Here we present rotamer inverted fragment finder–diffusion (Riff-Diff), a hybrid machine learning and atomistic modelling strategy for scaffolding catalytic arrays in de novo proteins. We highlight the general applicability of Riff-Diff by designing enzymes for two mechanistically distinct chemical transformations, the retro-aldol reaction and the Morita–Baylis–Hillman reaction. We show that in both cases, it is possible to generate catalysts that exhibit activities rivalling those optimized by in vitro evolution, along with exquisite stereoselectivity. High-resolution structures of six of the designs revealed near-atomic active site design precision.

We obtained crystal structures of the four designs: RAD13 (kcat = 3.8 × 10−5 s−1), RAD17 (kcat not determined), RAD32 (kcat = 1.1 × 10−2 s−1), and RAD36 (kcat = 6.2 × 10−5 s−1). The crystal structures agree with the design models, having backbone Cα RMSD values between 0.68 Å and 1.2 Å. In the active site of RAD36, we observed density for three distinct conformations of the catalytic lysine. One of the three lysine conformations points away from the active site, partially explaining its low catalytic rate. The observed alternative conformation of Y120 concomitant with the reduced activity of Y120F hints at a potential conformational change induced by substrate binding. Both results highlight how the prediction of activity needs to account for catalytic contributions beyond the interactions specified in the catalytic array and their conformational dynamics.

> SGMRERVEEALRRAKERREEIIGKYLEWAKTFANNPELQKEINERALKAIKDPSDEKDLKALGIALAIGMKGPIELGEEAVEELLGLLERLGKLSEKHAELADFLKALVQAYMTLKKTLSEEEYRVTYLGMIAVVLLALSEGDYDTAKAALELVVEGDYEPFLELAEPYAEEAKEAWEINKKLVEYGLKVLEKMKEAIKEVE3,4-DIMETHYLPHENOL | C8 H10 O 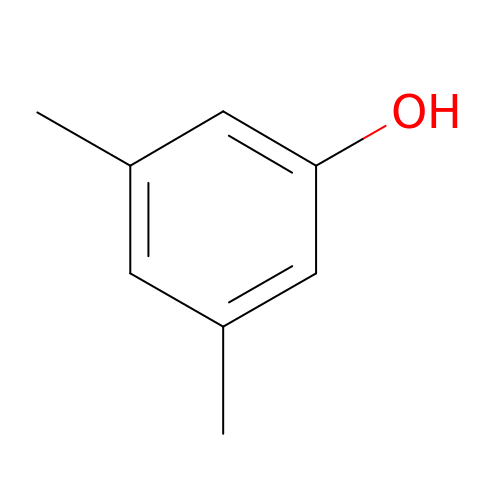| TUAMRELNJMMDMT-UHFFFAOYSA-N>[2x]MAHHHHHHMPLTDEEIANFKT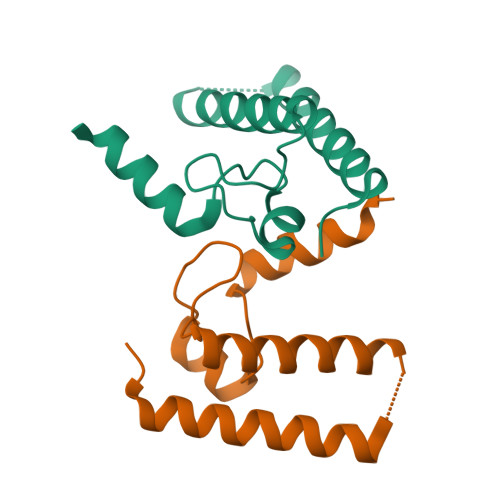RLLEMKAKLSHTLEGNAQEVKKPNEATGYSQHQADQGTDTFDRTISLEVTTKEYKLLRQIDRALEKIEEASYGICDVSGEEIPLARLMAIPYATMTVKSQEKFEKGLLSGN> MTVNWDINEALKNYMSDPSTIQTPEADSALVDCENDPESLLDNGLINSVLNPIVDAVAESPDAITRSHIFDSLQFLLKYTSYLSTHALSKLFDLITSGLGAEADVVHHDLESDEQELIPAHKQLLEMYGFLLQWTLTAAEAKAAEKSSTTVPARGRGKPKSKTGPGQDGTWDSVRQLETALSTMCKVLRLKLGKIFITTSERDTFIGLLTRPVYMILESEQRVKNTSIRMHAFKVLCMAVKHHGHGYAAQVSIVQNLTYFEHLSEPMAEFLHILAEQYDYPQLADEVLRELSNKEFNSNDTKGPKSVSAFMIRLSELAPRLVIKQVTLLAKQLDSESYTLRCALIEVFGNMLAYLSKSEERGENHKSQMNAFFDVLEERFLDINPYCRCRTIQVYIKLCELDQKFPKRRQRAAELACRSLMDKSSHVRRNAIKLLATLIRTHPFTALHGAQLARKDWQERLERVEAELNVLKPPPEAAGLEGDKANTSADQGLLDDATQVDSPKKRLEDMTEEEKIEAVRKAQEQAATSEAIEKLTLTKRYYTEALKFIDVLHEATPVICQLLGSKNKSEVIEAMDYFEIGDAYNIEQNKIGIRKMLRLIWTKGSSDEGKGVQTHLIECYKRLFFEAPDSFSPNDAANYIARNMISLTFGATPAELTSLEQLLHLMMKQGMIPDLVIAKLWQVYGVQRREISKKQRRGAIIVLGMLATASPEIVVGEMETMLRIGLGAHGRADLQLAKYTCIALRRINPTSRQTEKGSTTTFSRLPNDHAVLVKLAAITEVPTDNKEWYGVAEQAINAIYALSKHPDVLCSEIIRRKTRAVFARSTSKESVIGLSQLLFIVGHVAIKQIVHLELCELDFKRRKQEKDKEKAQQQEQEDNELDMIGGTTEDDFTEAMAHIRERELLFGPQSLLAQFGPMVSEICANNTVYKDRNLQQAATLCLAKLMCVSSEYCEANLPLLITIMERSPDPTVRSNAVIALGDMAVCFNHLIDENTDFLYRRLADPQPMVKRTCLMTLTFLILAGQVKVKGQLGEMAKCLEDEDKRIADLARMFFTELSTKDNAVYNHFVDMFSLLSADERIDEEAFRRIVRFLLGFVEKDKXXXXXXXXXXXXXXXXXXXXXXXXXXXXXXXXXXXXXXXXXXXXXXXXXXXXXX;> GHMED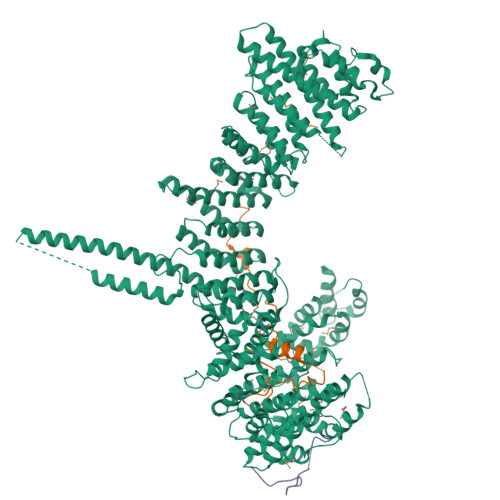GTVRKKPKKKTQRSSEATLAPSFASLQLKKLELEFAVDPFFKKASADFDEGGAKGLLLNHLMIDSQGRIVFDSSDDAEDVAEASAKPSREADDERPDSEDADADGDISMTDRDASAPGQVETQPEEEDEDVEIDVAALGAKYFPDLSILDSLDVCPSLKTFDLGDPSGSLYIPFLKVPDDWRHDQEKEKTPG> MTTTMKISIEFLEPFRMTKWQESTRRNKNNKEFVRGQAFARWHRNKKDNTKGRPYITGTLLRSAVIRSAENLLTLSDGKISEKTCCPGKFDTEDKDRLLQLRQRSTLRWTDKNPCPDNAETYCPFCELLGRSGNDGKKAEKKDWRFRIHFGNLSLPGKPDFDGPKAIGSQRVLNRVDFKSGKAHDFFKAYEVDHTRFPRFEGEITIDNKVSAEARKLLCDSLKFTDRLCGALCVIRFDEYTPAADSGKQTENVQAEPNANLAEKTAEQIISILDDNKKTEYTRLLADAIRSLRRSSKLVAGLPKDHDGKDDHYLWDIGKKKKDENSVTIRQILTTSADTKELKNAGKWREFCEKLGEALYLKSKDMSGGLKITRRILGDAEFHGKPDRLEKSRSVSIGSVLKETVVCGELVAKTPFFFGAIDEDAKQTALQVLLTPDNKYRLPRSAVRGILRRDLQTYFDSPCNAELGGRPCMCKTCRIMRGITVMDARSEYNAPPEIRHRTRINPFTGTVAEGALFNMEVAPEGIVFPFQLRYRGSEDGLPDALKTVLKWWAEGQAFMSGAASTGKGRFRMENAKYETLDLSDENQRNDYLKNWGWRDEKGLEELKKRLNSGLPEPGNYRDPKWHEINVSIEMASPFINGDPIRAAVDKRGTAVVTFVKYKAEGEEAKPVCAYKAESFRGVIRSAVARIHMEDGVPLTELTHSDCECLLCQIFGSEYEAGKI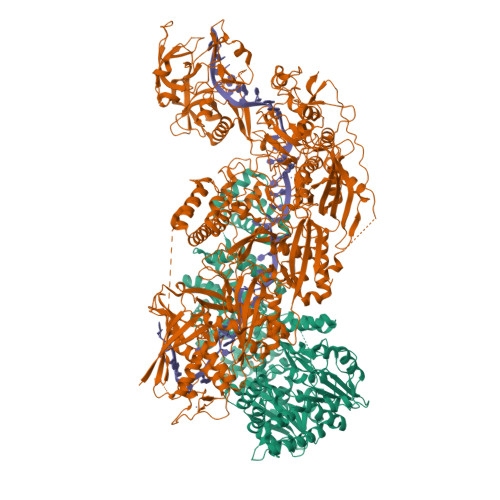RFEDLVFESDPEPVTFDHVAIDRFTGGAAAKKKFDDSPLPGSPARPLMLKGSFWIRRDVLEDEEYCKALGKALADVNNGLYPLGGKSAIGYGQVKSLGIKGDDKRISRLMNPAFDETDVAVPEKPKTDAEVRIEAEKVYYPHYFVEPHKKVEREEKPCGHQKFHEGRLTGKIRCKLITKTPLIVPDTSNDDFFRPADKEARKEKDEYHKSYAFFRLHKQIMIPGSELRGMVSSVYETVTNSCFRIFDETKRLSWRMDADHQNVLQDFLPGRVTADGKHIQKFSETARVPFYDKTQKHFDILDEQEIAGEKPVRMWVKRFIKRLSLVDPAKHPQKKQDNKWKRRKEGIATFIEQKNGSYYFNVVTNNGCTSFHLWHKPDNFDQEKLEGIQNGEKLDCWVRDSRYQKAFQEIPENDPDGWECKEGYLHVVGPSKVEFSDKKGDVINNFQGTLPSVPNDWKTIRTNDFKNRKRKNEPVFCCEDDKGNYYTMAKYCETFFFDLKENEEYEIPEKARIKYKELLRVYNNNPQAVPESVFQSRVARENVEKLKSGDLVYFKHNEKYVEDIVPVRISRTVDDRMIGKRMSADLRPCHGDWVEDGDLSALNAYPEKRLLLRHPKGLCPACRLFGTGSYKGRVRFGFASLENDPEWLIPGKNPGDPFHGGPVMLSLLERPRPTWSIPGSDNKFKVPGRKFYVHHHAWKTIKDGNHPTTGKAIEQSPNNRTVEALAGGNSFSFEIAFENLKEWELGLLIHSLQLEKGLAHKLGMAKSMGFGSVEIDVESVRLRKDWKQWRNGNSEIPNWLGKGFAKLKEWFRDELDFIENLKKLLWFPEGDQAPRVCYPMLRKKDDPNGNSGYEELKDGEFKKEDRQKKLTTPWTPWASSGLVPRGSHHHHHHH;> MSNPIRDIQDRLKTAKFDNKDDMMNLASSLYKYEKQLMDSSEATLCQQGLSNRPNSFSQLSQFRDSDIQSKAGGQTGKFWQNEYEACKNFQTHKERRETLEQIIRFLQNGAEEKDADDLLLKTLARAYFHRGLLYRPKGFSVPARKVEAMKKAIAYCEIILDKNEEESEALRIWLYAAMELRRCGEEYPENFAEKLFYLANDGFISELYDIRLFLEYTEREEDNNFLDMILQENQDRERLFELCLYKARACFHLNQLNDVRIYGESAIDNAPGAFADPFWDELVEFIRMLRNKKSELWKEIAIKAWDKCREKEMKVGNNIYLSWYWARQRELYDLAFMAQDGIEKKTRIADSLKSRTTLRIQELNELRKDAHRKQNRRLEDKLDRIIEQENEARDGAYLRRNPPCFTGGKREEIPFARLPQNWIAVHFYLNELESHEGGKGGHALIYDPQKAEKDQWQDKSFDYKELHRKFLEWQENYILNEEGSADFLVTLCREIEKAMPFLFKSEVIPEDRPVLWIPHGFLHRLPLHAAMKSGNNSNIEIFWERHASRYLPAWHLFDPAPYSREESSTLLKNFEEYDFQNLENGEIEVYAPSSPKKVKEAIRENPAILLLLCHGEADMTNPFRSCLKLKNKDMTIFDLLTVEDVRLSGSRILLGACESDMVPPLEFSVDEHLSVSGAFLSHKAGEIVAGLWTVDSEKVDECYSYLVEEKDFLRNLQEWQMAETENFRSENDSSLFYKIAPFRIIGFPAE>GSSHHHHHHSSGLVPRGSHMASSADDDGIDDVQEEEEEQPVEPGEEEDDEVADWGEVAENLQEQTYNIYLTSNGTFRQDNEGNENFNYWWNAHMLDVLIDGYERTGDESYLPKMKSLLEGIEVRNGNKYENVFIDDMEWLGIACLRTYKLTNDQQYKEVADLLWEETKQGWSDVHGGGIAWKTDTPNSKNACSNGPAAIFALYLYEIDQDEEDLEWAKKIYHWLKDTLVDPESGLVWDNIDYHDGEAIINRDWIFTYNVGTYIGAANLLHQATGEGMYLDDAIKSASSVVAPGELTTGGVLKNEGQGDGGLFKGILVRYFTQLALNPDLPDGKRNEFEEFVLFNAETLYHNGLTSAGLAGPNWNDEPSGRVDLS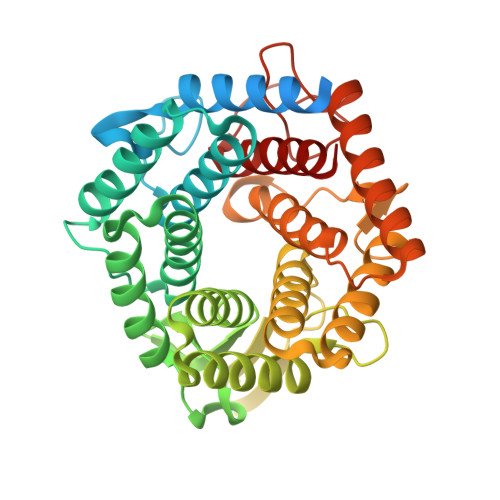TQLSGVMLMEAKALLE[3x]In this work, we report the crystal structures of porcine b5 determined at sub-angstrom resolutions in both the oxidized and reduced forms. The haem Fe atom is coordinated by two axial ligands, His44 and His68, and the haem group is not bound covalently to the protein moiety. The haem orientation in porcine b5 corresponds to the major isomer observed in the rat b5 structure. The comparison using high-resolution structures revealed that structural differences around the haem group may be important for regulating the electronic properties of the haem.

The crystal structures were determined at resolutions of 0.83 Å (oxidized form 1), 0.93 Å (oxidized form 2), 0.76 Å (reduced form 1) and 0.95 Å (reduced form 2). Form 1 and 2 crystals were obtained at pH 7.4 and 5.5, respectively. One of the Ca2+ ions (Ca-1) is coordinated by the side-chain carboxyl groups of two glutamic acid residues, Glu42 and Glu48, located around the axial ligand His44. On the other hand, the uniform C—O distances in the oxidized form 1 structure indicate that the 7-propionate group is in a charged state. Unrestrained refinement was also applied to the 6-propionate group in the oxidized form 1 structure. The C—O1 [1.253 (9) Å] and C—O2 [1.246 (10) Å] distances are consistent with the results for the 7-propionate group. The hydrogen-bond distance from His68 Nδ1 to Phe63 O is 2.893 (6) Å in the oxidized form 1 structure and 3.097 (5) Å in the reduced form 1 structure. The interactions with Arg89* and other interactions with the neighbouring molecules in the crystal fix the structure from Phe63 to His68, and small spaces exist between the adjacent molecules. In addition, water molecules were found near the main-chain atoms of Phe63 and His68 in the form 1 structures. The water molecules form hydrogen bonds to both the main-chain carbonyl of Phe63 and the main-chain amide of His68. The hydrogen-bond distances in the oxidized form 1 structure are shorter (0.2–0.4 Å) than those in the reduced form 1 structure.

> MAEQSDKAVKYYTLEEIQKHNNSKSTWLILHHKVYDLTKFLEEHPGGEEVLREQAGGDATENFEDVGHSTDARELSKTFIIGELHPDDRSKIAK> EPEWTYPRLSCQGSTFQKALLISPHRFGEIKGNSAPLIIREPFVACGPKECRHFALTHYAAQPGGYYNGTRKDRNKLRHLVSVKLGKIPTVENSIFHMAAWSGSACHDGREWTYIGVDGPDNDALVKIKYGEAYTDTYHSYAHNILRTQESACNCIGGDCYLMITDGSASGISKCRFLKIREGRIIKEILPTGRVEHTEECTCGFASNKTIECACRDNSYTAKRPFVKLNVETDTAEIRLMCTKTYLDTPRPDDGSIAGPCESNGDKWLGGIKGGFVHQRMASKIGRWYSRTMSKTNRMGMELYVRYDGDPWTDSDALTLSGVMVSIEEPGWYSFGFEIKDKKCDVPCIGIEMVHDGG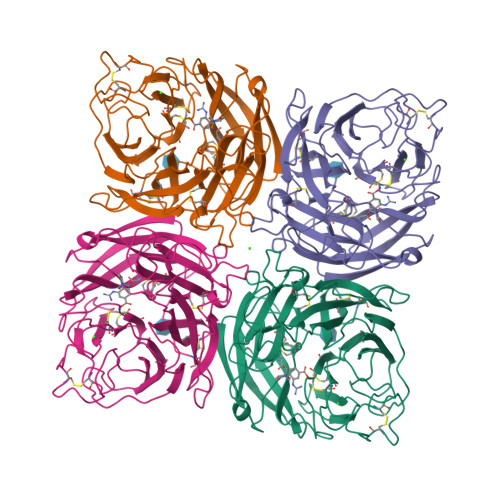KDTWHSAATAIYCLMGSGQLLWDTVTGVDMAL The nucleoside proton symporter (NHS) family proteins are part of the major facilitator superfamily and are responsible for transporting nucleosides from the extracellular environment into the cell. In this study, using X-ray crystallography, molecular dynamics simulations, and biochemical assays, we discovered that the deprotonation of Asp323 in NupG, or the equivalent Asp315 in YegT, (another NHS family member) triggers a local conformational change in the TM10 region of NHS transporters. Notably, this protonation site is part of a novel motif (GXXXD) located in the middle of the TM10 transmembrane helix in NHS proteins. Further biochemical studies suggest that this local conformational change in the GXXXD motif plays a role in coordinating substrate release, ultimately facilitating substrate translocation.

We introduced a point mutation in YegT (YegTK267A) to improve the quality of the crystal and crystallized the protein using the lipidic cubic phase method. Through molecular replacement, we determined the structure of YegTK267A at a resolution of 3.1 Å. The asymmetric unit, contained two YegT molecules, designated as molecule A and molecule B. Notably, both molecules were captured in nearly identical conformations, with a RMSD of 0.17 Å across 332Cα atoms. Notably, Lys267 is located in the loop connecting TM8 and TM9, which is distant from the substrate-binding site. This placement ensures that the mutation has minimal effect on the substrate-binding region. A structural comparison between two NHS members, NupG and YegT, revealed that both proteins share similar structural features, with an RMSD of approximately 1.57 Å across 316 Cα atoms, despite having only about 27% sequence identity. The protonation site, Asp315 in YegT, and the corresponding residue Asp323 in NupG, are situated within this conserved motif. Given that the measured pH obtained for the crystallization condition was 5.8, this strongly suggests that Asp315 is protonated. Notably, the side-chain carbonyl oxygen atom of Asp315 is located solely 2.5 Å apart of the main-chain carbonyl oxygen atom of Glu255.

>[2x]MKTTAKLSFMMFVEWFIWGAWFVPLWLWLSKSGFSAGEIGWSYACTAIAAILSPILVGSITDRFFSAQKVLAVLMFAGALLMYFAAQQTTFAGFFPLLLAYSLTYMPTIALTNSIAFANVPDVERDFPRIRVMGTIGWIASGLACGFLPQILGYADISPTNIPLLITAGSSALLGVFAFFLPDTPPKSTGKMDIKVMLGLDALILLRDKNFLVFFFCSFLFAMPLAFYYIFANGYLTEVGMKNATGWMTLGQFSEIFFMLALPFFTARFGIKKVLLLGLVTAAIRYGFFIYGSADEYFTYALLFLGILLHGVSYDFYYVTAYIYVDKKAPVHMRTAAQGLITLCCQGFGSLLGYRLGGVMMEKMFAYQEPVNGLTFNWSGMWTFGAVMIAIIAVLFMIFFRESDNEITAIKVDDRDIALTQGEVK>MKNAPSTAGGGYGSWEIDPKDLTFLKELGTGQFGVVKYGKWRGQYDVAIKMIREGSMSEDEFIEEAKVMMNLS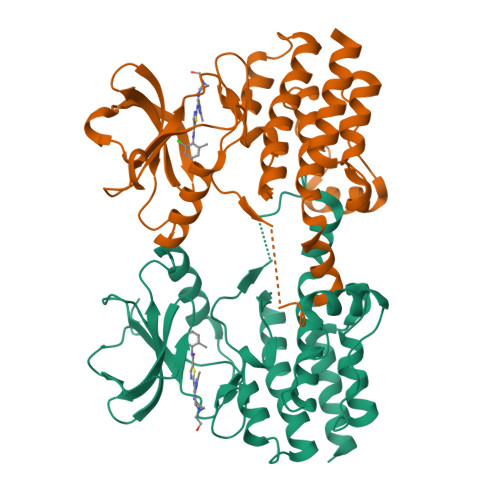HEKLVQLYGVCTKQRPIFIITEYMANGCLLNYLREMRHRFQTQQLLEMCKDVCEAMEYLESKQFLHRDLAARNCLVNDQGVVKVSDFGLSRYVLDDEETSSVGSKFPVRWSPPEVLMYSKFSSKSDIWAFGVLMWEIYSLGKMPYERFTNSETAEHIAQGLRLPRPHLASERVYTIMYSCWHEKADERPSFKILLSNILDVMDEES[2x]6-(3-bromophenyl)pteridine-2,4,7-triamine | C12 H10 Br 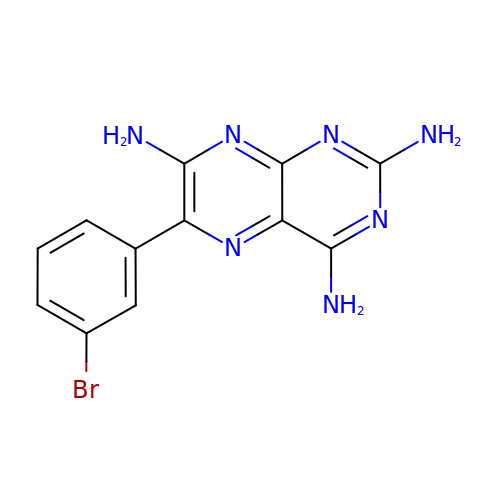N7 | UWFFWZGQGRBIBG-UHFFFAOYSA-N>[3x]SNAVVQRAAETYDLLKQRTEELRRANAQMSLLTVLVQVTQASNSLEAILTPIATAFA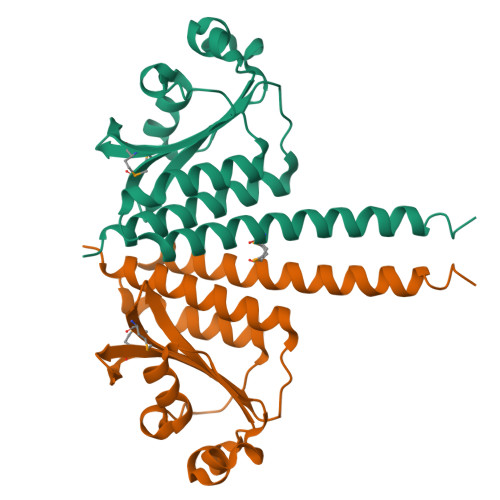ESFAVNACILQMLEGQTLSTIQGFYSQQGTVNNWLNQDPLTNEAIATGQIQVAANIAKDPKLASISQYQDNGIQSHVVIPITYRNEMLGVLSLQWQQPISLREDELTLIHLSAQLVAIALTSSRCSL>GSHMSLIDPRAIIDPSARLAADVQVGPWSIVGAEVEIGEGTVIGPHVVLKGPTKIGKHNRIYQFSSVGEDTPDLKYKGEPTRLVIGDHNVIREGVTIHRGTVQDRAETTIGDHNLIMAYAHIGHDSVIGNHCILVNNTALAGHVHVDDWAILSGYTLVHQYCRIGAHSF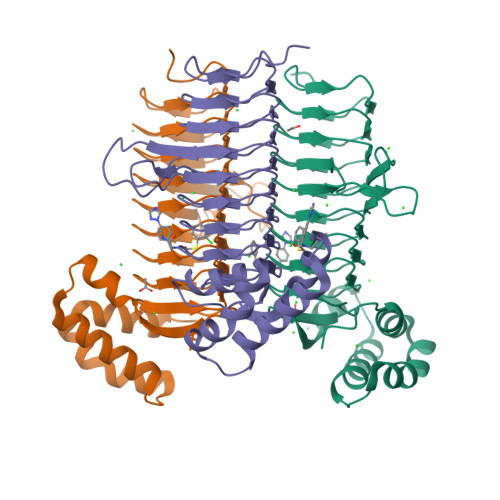SGMGSAIGKDVPAYVTVFGNPAEARSMNFEGMRRRGFSSEAIHALRRAYKVVYRQGHTVEEALAELAESAAQFPEVAVFRDSIQSATRGITR[3x]>[2x]DELAFSPPFYPSPWANGQGEWAEAYQRAVAIVSQMTLDEKVNLTTGTGWELEKCVGQTGGVPRLNIGGMCLQDSPLGIRDSDYNSAFPAGVNVAATWDKNLAYLRGQAMGQEFSDKGIDVQLGPAAGPLGRSPDGGRNWEGFSPDPALTGVLFAETIKGIQDAGVVATAKHYILNEQEHFRQVAEAAGYGFNISDTISSNVDDKTIHEM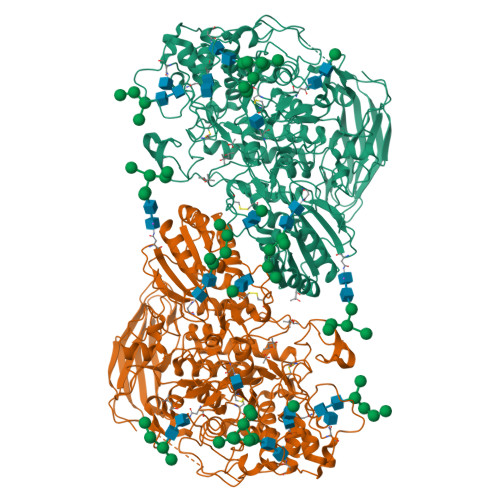YLWPFADAVRAGVGAIMCSYNQINNSYGCQNSYTLNKLLKAELGFQGFVMSDWGAHHSGVGSALAGLDMSMPGDITFDSATSFWGTNLTIAVLNGTVPQWRVDDMAVRIMAAYYKVGRDRLYQPPNFSSWTRDEYGFKYFYPQEGPYEKVNHFVNVQRNHSEVIRKLGADSTVLLKNNNALPLTGKERKVAILGEDAGSNSYGANGCSDRGCDNGTLAMAWGSGTAEFPYLVTPEQAIQAEVLKHKGSVYAITDNWALSQVETLAKQASVSLVFVNSDAGEGYISVDGNEGDRNNLTLWKNGDNLIKAAANNCNNTIVVIHSVGPVLVDEWYDHPNVTAILWAGLPGQESGNSLADVLYGRVNPGAKSPFTWGKTREAYGDYLVRELNNGNGAPQDDFSEGVFIDYRGFDKRNETPIYEFGHGLSYTTFNYSGLHIQVLNASSNAQVATETGAAPTFGQVGNASDYVYPEGLTRISKFIYPWLNSTDLKASSGDPYYGVDTAEHVPEGATDGSPQPVLPAGGGSGGNPRLYDELIRVSVTVKNTGRVAGDAVPQLYVSLGGPNEPKVVLRKFDRLTLKPSEETVWTTTLTRRDLSNWDVAAQDWVITSYPKKVHVGSSSRQLPLHAALPKVQ> MQALRRGAAIPSRLLPRRDSWMSLAPFVAPNNAAAWRKLRDGAQEVQTVIERQSTPGKPQQIDWAKWESQIAHKDILNCLKTFYTNQVQILDRALGALETAKTPAPCEGAEKGWALFDAALSACAKSVEKSEELLSNGARALWVSCSNPPVWKVNTNEWLDSDQYWQAFVEKHHFYSQYQPGVVDPEAPQEVEAFKQAWHSRMGKFNDRSDTPMLYAYMNELPSWEYYDLHRSAFLEHMTYFLVRTGGDFRFFPEMPPWQWLAHMENLRFKLLSVAQSRRSQLQLANLERERALDFLPVDVEHHGEEYTQKFLQYETELFQACAARLMGHFMFLCDPFIPVQSAEALSAVTRVDNGKGKLFSLGDDVNALFYLPEQQRRDVERPTQAVQTLLGHLEATGRPFNPCYSELLHVHAEVLEERGEHWLTAPGECVSQAFLRRLRTDDPAYEVYCSYFKEMYERFAGAKEVSMEDGRKRLATIEKNAQEEAAAYGLALKTMGSAELAHKAREGAAKLEQLRKAQEKAAGKSAQTVQENKM;> MNFSSSARWLAVRQSQTLGHTTRATVAAGRRVLAHSPAATEFTSFQSLHIGGDVCKLPLAVALGAAPSALGYGSAKHNQQRQYATLGSGWSFSKVQYTKYRITKPWTTDTTFDDIILSQPSKEDFAKFTKEAPLFLRFLKLVTDVEGRQEAFIQFAKRCENGLTVEKDVYVTKKELVDCLWKNGYTDTEINAFEIAFPADYKFHYPELAVLFDLTEEDCYK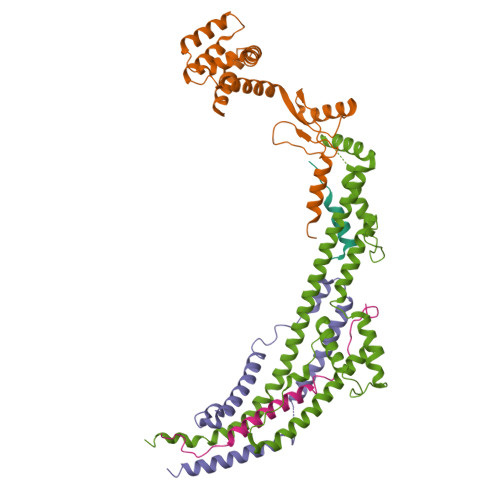YCIRQRAATPEELVELKYTKPKNLVSSYGLCFLGVWFGLSNTVLSNAWFYSKTFPFGAVFYMLGSYFYRDIREKLWKEEKSLIHTAQENKNMGEESVYKQMKKYATDTKCLDYLSTFRTEVEDQIANYKVALVSQMRRQLTERLVEKLNGIQQAEKLIQGSLQDVMIREIVSSFKDLYKSRPELHDAAMQSAIQGLSGSDGAMDPVGAHFKASLQELAKVNLSTATADPMGTVVQRVAAVFQKREKEFLDTFTVKATEAQEIKTIVDKCHKGNTFDFHALSDEELRRLEQLYSTVNNRVGFETIHENSIKPVAPLSENSKGFVEFVNTQLEITKAKLRNARLTAFAHAFV;> MTIHSCLARRAVSVAASGARAFASGLGARAVAVGALQSARLLHTSSLRAAGAKISPSEMSRLLEERIAGWKTQTSTEEVGRVVSVGDGIARLFGLEGVQAGELVEFQNGMTGMALNLETDNVGVVIFGDDRSVLEGDSVKRTGRIVDVPIGPGLLGRVVDALGNPIDGKGPIPAKERRRVELKAPGIIPRKSVHEPMMTGLKCVDALVPVGRGQRELIIGDRQTGKTAVAVDAIINQKEINDSTDDESKKLYCIYVAVGQKRSTVAQIVKALEQRDAMKYTTVVAATASEAAPLQFLAPYSGCAMGEWFRDSGRHCVIIYDDLSKQATAYRQMSLLLRRPPGREAYPGDVFYLHSRLLERAAKMGDKSGGGSLTALPVIETQAGDVSAYIPTNVISITDGQIFLETELFYKGIRPAINVGLSVSRVGSAAQVKAMKQVAGTMKLELAQYREVAAFAQFGSDLDASTRQLLTRGTALTELLKQRQYSPMKNSVQVCVLYCGVKGYLDPLDPKEISRFESLFIDYINANHQDILKTIETEKELSEKTEAKLRAAVDEFVAMNEFKKK;> MALPLLASRRLFSSFVFRGQPSTLSSNLSLVRIRGLHGGSLSPPSATLPRAVQLFSSRIAFSTAAAEDSGASQTLEGRYASALFRVAKKKNQLEKVYGDLESVRNALKDSSEFRLFVDSPAVSVQQKLDVLRQLVNRYKFDPLTGNLLTTLVENKRLPMLARVADAFDAMYRKEKGEVKCLVTSAKPLSAQQQKEIVAALQNRAGTQARLIIDYAVSPQIMGGLVVRLGEQVLDFSVATRLDRLQSQLLAPL;> MLNFIPKRCPSVSLLFGKRPVQRIEVGQARHQLEIPVETIEKIYEGVDSRLEYHNKDYNAMKWKDFMKLKLDAYHLLEASQSETAAKSALSDLNWFSDLADIYSGQQTMAEMDVALKAQGEQKLSYPIQGKNIK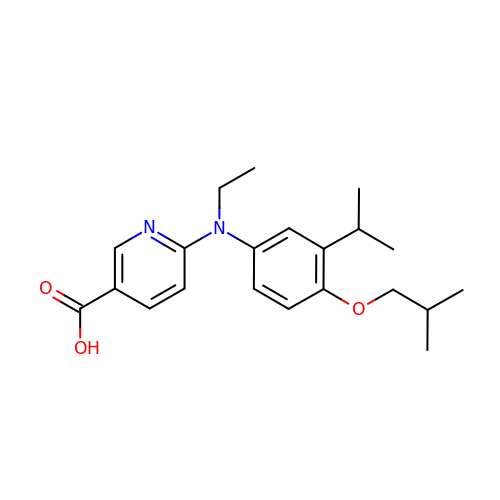6-[ethyl-[4-(2-methylpropoxy)-3-propan-2-yl-phenyl]amino]pyridine-3-carboxylic acid | C21 H28 N2 O3 | QNFFQLHRCGJHHN-UHFFFAOYSA-N>SLGLQDFDLLRVIGRGSYAKVLLVRLK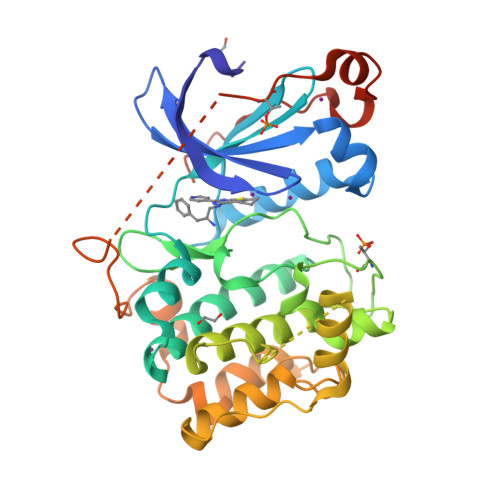KTDRIYAMKVVKKELVNDDEDIDWVQTEKHVFEQASNHPFLVGLHSCFQTESRLFFVIEYVNGGDLMFHMQRQRKLPEEHARFYSAEISLALNYLHERGIIYRDLKLDNVLLDSEGHIKLTDYGMCKEGLRPGDTTSTFCGTPNYIAPEILRGEDYGFSVDWWALGVLMFEMMAGRSPFDIVGSSDNPDQNTEDYLFQVILEKQIRIPRSLSVKAASVLKSFLNKDPKERLGCHPQTGFADIQGHPFFRNVDWDMMEQKQVVPPFKPNISGEFGLDNFDSQFTNEPVQLTPDDDDIVRKIDQSEFEGFEYINPLLMSAEESV[3x]>[2x]IGDEPLENYLDTEYFGTIGIGTPAQDFTVIFDTGSSNLWVPSVYCSSLACSDHNQFNPDDSSTFEATSQELSITYGTGSMTGILGYDTVQVGGISDTNQIFGLSETEPGSFLYYAPFDGILGLAYPSISASGATPVFDNLWDQGLVSQDLFSVYLSSNDDSGSVVLLGGIDSSYYTGSLNWVPVSVEGYWQITLDSITMDGETIACSGGCQAIVDTGTSLLTGPTSA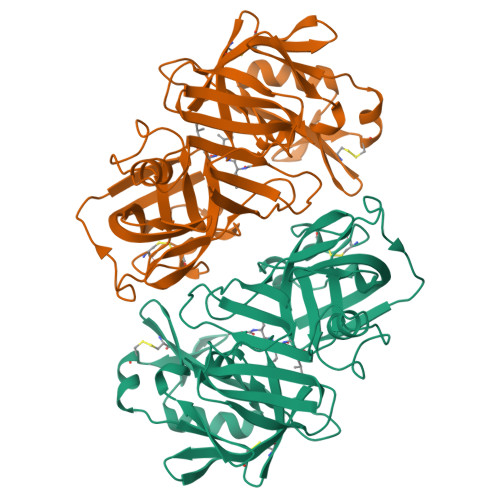IANIQSDIGASENSDGEMVISCSSIDSLPDIVFTINGVQYPLSPSAYILQDDDSCTSGFEGMDVPTSSGELWILGDVFIRQYYTVFDRANNKVGLAPVA DIBENZOFURAN | C12 H8 O | 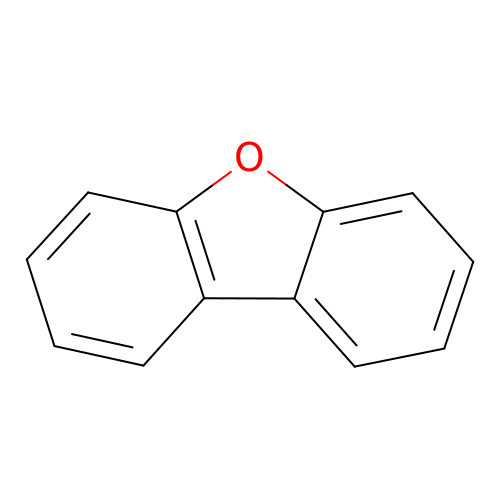TXCDCPKCNAJMEE-UHFFFAOYSA-N> SMQFSKMHGLGNDFMVVDAVTQNVFFSPELIRRLADRHLGVGFDQLLVVEPPYDPELDFHYRIFNADGSEVAQCGNGARCFARFVRLKGLTNKRDIRVSTANGRMVLTVTDDDLVRVNMGEPNFEPSAVPFRANKAEKTYIMRAAEQTILCGVVSMGNPHCVIQVDDVDTAAVETLGPVLESHERFPERANIGFMQVVKREHIRLRVYERGAGETQACGSGACAAVAVGIQQGLLAEEVRVELPGGRLDIAWKGPGHPLYMTGPAVHVYDGFIHL;> SMIDDDGYRPNVGIVICNRQGQVMWARRFGQHSWQFPQGGINPGESAEQAMYRELFEEVG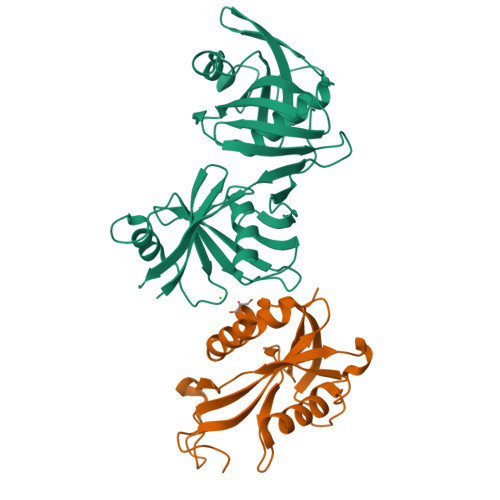LSRKDVRILASTRNWLRYKLPKRLVRWDTKPVCIGQKQKWFLLQLVSGDAEINMQTSSTPEFDGWRWVSYWYPVRQVVSFKRDVYRRVMKEFASVVMSLQ> SSKEVAELKKQVESAELKNQRLKEVFQTKIQEFRKACYTLTGYQIDITTENQYRLTSLYAEHPGDCLIFKATSPSGSKMQLLETEFSHTVGELIEVHLRRQDSIPAFLSSLTLELFSRQTV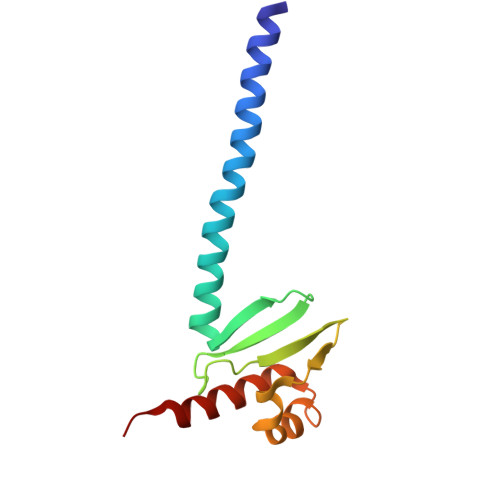A>GPAASAGRIERRRARAAVAGRDATGRFTAGQPRRVELDADATSGAFYARYRDGYVSGEPWPGAGPPPPGRVLYGGLGDSRPGLWGAPEAEEARRRFEASGAPAAVWAPELGDAAQQYALITRLLYTPDAEAMGWLQNPRVVPGDVALDQACFRISGAARNSSSFITGSVARAVPHLGYAMAAGRFGWGLAHAAAAVAMSRRYDRAQKGFLLTSLRRAYAPLLARENAALTG[4x];> FTA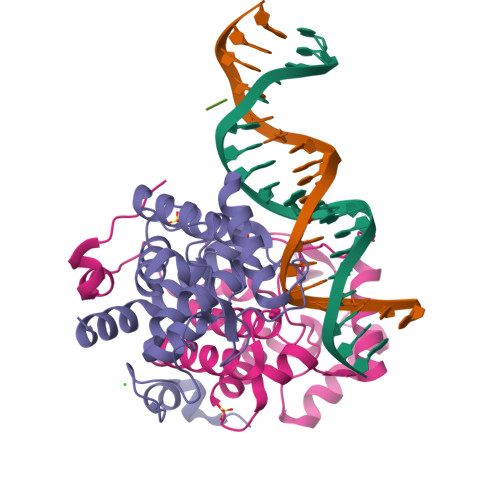G VanS is a sensor histidine kinase that responds to the presence of vancomycin by autophosphorylating and subsequently transferring the phosphoryl group to the response regulator, VanR. The phosphotransfer activates VanR as a transcription factor, which initiates the expression of resistance genes. The VanS sensor kinase is organized into several structural domains, which include a periplasmic sensor domain flanked by two transmembrane helices, a membrane-proximal HAMP domain, a dimerization-and-histidine-phosphorylation (DHp) domain, and a catalytic ATP-binding (CA) domain. Here, we present X-ray crystal structures for the catalytic and ATP-binding (CA) domains of two VanS proteins, derived from vancomycin-resistant enterococci types A and C. Both proteins adopt the canonical Bergerat fold that has been observed for CA domains of other prokaryotic histidine kinases.

The structure of the VanSA CA domain was determined by the single-wavelength anomalous diffraction method, relying upon two ordered cadmium ions contributed by the crystallization buffer. The crystal asymmetric unit contains one copy of the CA domain, and the cadmium ions mediate two of the three lattice contacts that connect different VanSA molecules within the crystal. The structure was refined separately against two different data sets, one of which was measured at low energy (7 keV) and used for phasing, whereas the other was collected at an energy more typically used for protein crystallography (13.5 keV). The structures obtained from the two different data sets are essentially identical, with a few minor differences in side-chain conformers, and have an RMSD in Cα positions of 0.14 Å (0.59 Å for all nonhydrogen atoms). In particular, helix α3 occupies very different positions in the two structures, being positioned much closer to the nucleotide-binding site in VanSA than in VanSC. Notably, α3 is involved in a crystal contact in the VanSA crystals, packing against strand β5 in a neighboring molecule in the lattice. Were α3 to occupy the same position in the VanSA structure that it does in the VanSC structure, it would clash with the symmetry-related molecule. Hence, it seems likely that the ATP lids of VanSA and VanSC can adopt a range of positions, and crystallization of these two proteins has selected for two different conformers. VanSA is an exception, as its α3 helix lies closer to the nucleotide-binding site than in any of the other proteins; this likely reflects crystal packing effects.

> NLQTITLTKTHIDLYYMLVQMTDEFYPQLSAHGKQAVIHAPEDLTVSGDPDKLARVFNNILKNAAAYSEDNSIIDITAGLSGDVVSIEFKNTGSIPKDKLAAIFEKFYRLDNARSSDTGGAGLGLAIAKEIIVQHGGQIYAESNDNYTTFRVELPAMPDLVDKRRS S-(DIFLUOROMETHYL)HOMOCYSTEINE | C5 H9 F2 N O2 S | 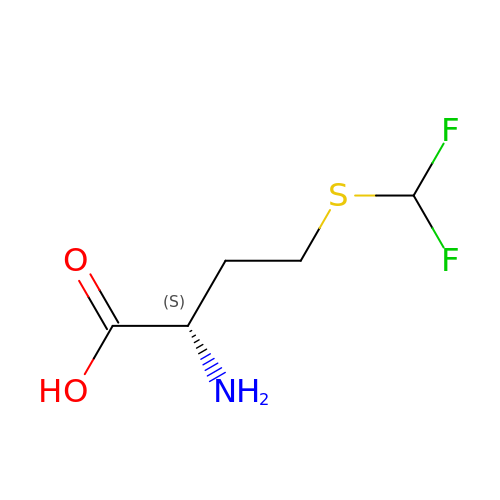YHBNXKYHZMAFED-VKHMYHEASA-N3'-DEOXY-3'-ACETAMIDO-THYMIDINE | C12 H17 N3 O5 | 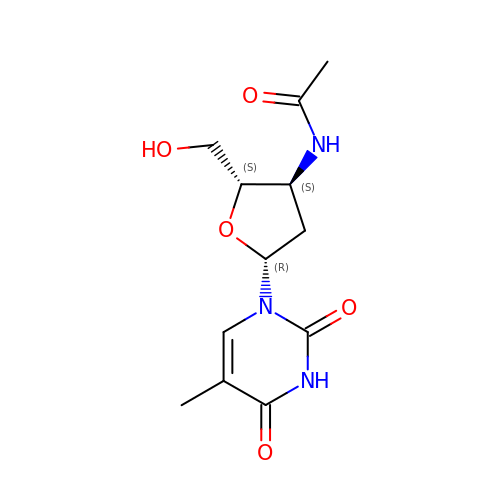OCWNRLPPKHGFCE-IVZWLZJFSA-N>[18x]MSQYSIQQSLGNASGVAVSPINADATLSTGVALNSSLWAGIGVFARGKPFTVLAVTESNYEDVLGEPLKPSSGSQFEPIRHVYEAIQQTSGYVVRAVPDDAKFPIIMFDESGEPAYSALPYGSEIELDSGEAFAIYVDDGDPCISPTRELTIETATADSAGNERFLLKLTQTTSLGVVTTLETHTVSLAEEAKDDMGRLCYLPTALEARSKYLRAVVNEELISTAKVTNKKSLAFTGGTNGDQSKISTAAYLRAVKVLNNAPYMYTAVLGLGCYDNAAITALGKICADRLIDGFFDVKPTLTYAEALPAVEDTGLLGTDYVSCSVYHYPFSCKDKWTQSRVVFGLSGVAYAAKARGVKKNSDVGGWHYSPAGEERAVIARASIQPLYPEDTPDEEAMVKGRLNKVSVGTSGQMIIDDALTCCTQDNYLHFQHVPSLMNAI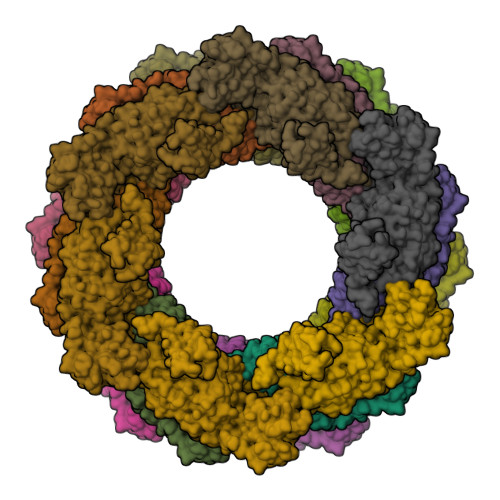SRFFVQLARQMKHSPDGITAAGLTKGMTKLLDRFVASGALVAPRDPDADGTEPYVLKVTQAEFDKWEVVWACCPTGVARRIQGVPLLIK> MDSPSSLHIAMFPWFAMGHLIPYLHLSNKLAKRGHKISFFTPKKTQTKLEQFNLYPNLITFYPLNVPHVDGLPFGAETTSDVAISLGPILMTAMDQTQNQIELLLTQLKPQIIFFDFVFWLPKITQRLGIKSFLYFIINPATISYTTSPPRMFEAENLTEVDLMKPPKGYPTSFNLQSHEAKHLASTRKIEFGSGIPFSVRSYNCLSLTDAIGFKGCREIEGPYVDYLQEQFGKPVLLSGPVLPEQSKTALDEKW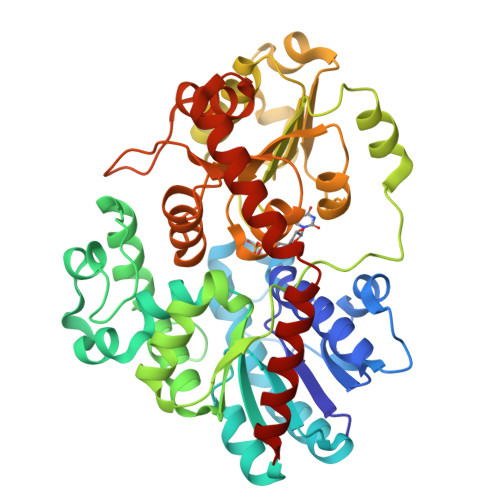GSWLGGFKDGSLVYCALGSELKLKQDQFHELLLGLELTGFPFLAILKPPVGFETIEDALPEGFKERVKEKGIVHSGWIQQQLILEHPSVGCFVTHCGAGSITEGLVNNCQMVLLPQLNGDYIINARIMGRHLKVGVEVKKGEEDGLFTKESVYEAVKIVMDDENEIGREVRSNHTKVRNLLLRHDLESSCLDTFCEKLQELVS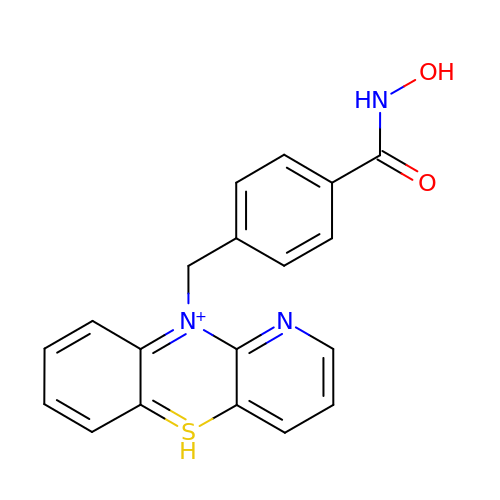10-{[4-(hydroxycarbamoyl)phenyl]methyl}-5lambda~4~-pyrido[3,2-b][1,4]benzothiazin-10-ium | C19 H16 N3 O2 S | AIQWDXVAECMLSN-UHFFFAOYSA-O>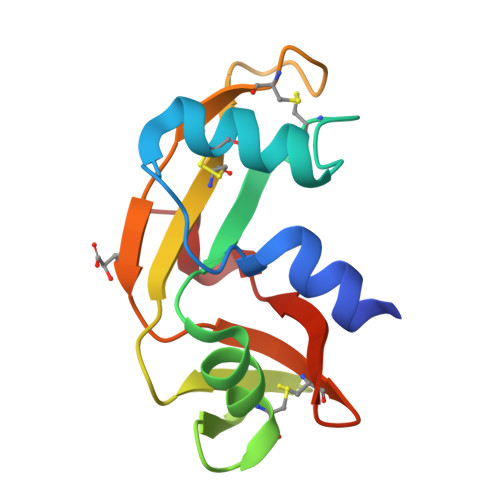 QDNSRYTHFLTQHYDAKPQGRDDRYCESIMRRRGLTSPCKDINTFIHGNKRSIKAICENKNGNPHRENLRISKSSFQVTTCKLHGGSPWPPCQYRATAGFRNVVVACENGLLVHLDQSIFRRP> GLIVDTRDVEERVHVMRKTKLAPTVAHGVFNPEFGPAALSNKDPRLN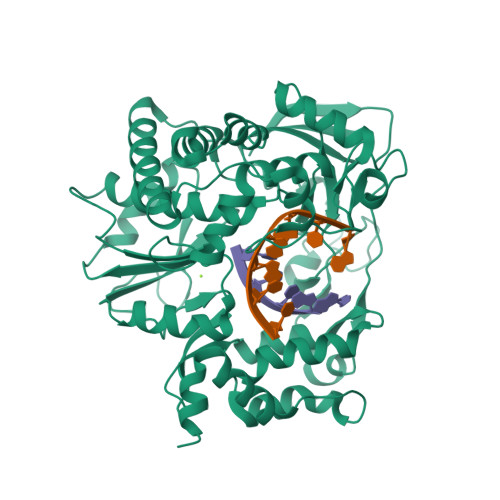EGVVLDEVIFSKHKGDTKMSAEDKALFRRCAADYASRLHSVLGTANAPLSIYEAIKGVDGLDAMEPDTAPGLPWALQGKRRGALIDFENGTVGPEVEAALKLMEKREYKFACQTFLKDEIRPMEKVRAGKTRIVDVLPVEHILYTRMMIGRFCAQMHSNNGPQIGSAVGCNPDVDWQRFGTHFAQYRNVWDVDYSAFDANHCSDAMNIMFEEVFRTEFGFHPNAEWILKTLVNTEHAYENKRITVEGGIPSGCSATSIINTILNNIYVLYALRRHYEGVELDTYTMISYGDDIVVASDYDLDFEALKPHFKSLGQTITPADKSDKGFVLGHSITDVTFLKRHFHMDYGTGFYKPVMASKTLEAILSFARRGTIQEKLISVAGLAVHSGPDEYRRLFEPFQGLFEIPSYRSLYLRWVNAVCGDAAALEHH>[2x]GPSFWLGNETLKVPLALFALNRQRLCERLRKNP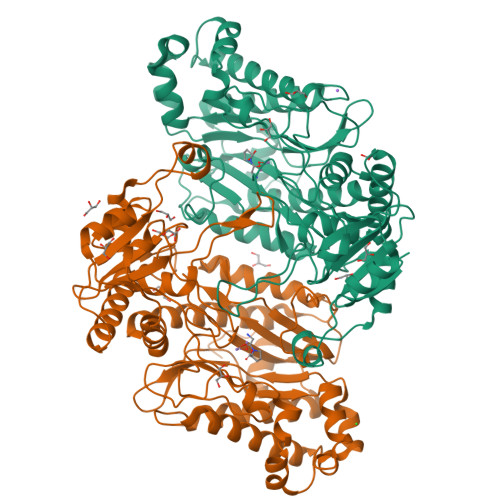AVQAGSIVVLQGGEETQRYCTDTGVLFRQESFFHWAFGVTEPGCYGVIDVDTGKSTLFVPRLPASHATWMGKIHSKEHFKEKYAVDDVQYVDEIASVLTSQKPSVLLTLRGVNTDSGSVCREASFDGISKFEVNNTILHPEIVECRVFKTDMELEVLRYTNKISSEAHREVMKAVKVGMKEYELESLFEHYCSRGGMRHSSYTCICGSGENSAVLHYGHAGAPNDRTIQNGDMCLFDMGGEYYCFASDITCSFPANGKFTADQKAVYEAVLRSSRAVMGAMKPGVWWPDMHRLADRIHLEELAHMGILSGSVDAMVQAHLGAVFMPHGLGHFLGIDVHDVGGYPEGVERIDEPGLRSLRTARHLQPGMVLTVEPGIYFIDHLLDEALADPARASFLNREVLQRFRGFGGVRIEEDVVVTDSGIELLTCVPRTVEEIEACMAGCDKAF~{tert}-butyl ~{N}-[(2~{S})-2-methyl-4-oxidanyl-1-oxidanylidene-pent-4-en-2-yl]carbamate | C11 H19 N O4 | 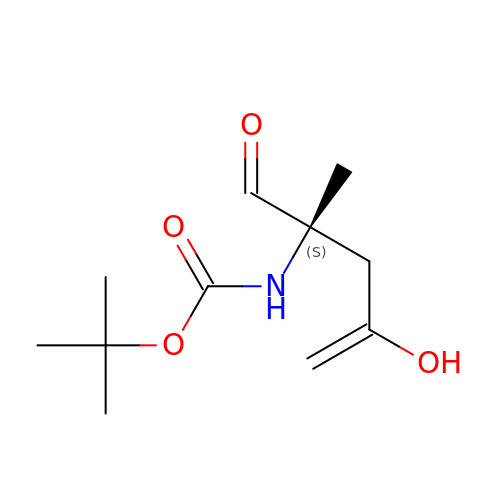DGQSAFHPNXJDHT-NSHDSACASA-N> SLQQPEWQSQYAVGLNKLDPHTYVWPYADASEVEKGTFEQSPYYMSLNGQWKFHWVKNPDTRPKDFYKPSYYTGGWADIKVPGNWERQGYGTAIYVNETYEFDDKMFNFKKNPPLVPYKENEVGSYRRTFKVPAGWEGRRVVLCCEGVISFYYVWVNGEFLGYNQGSKTAAEWDITDKLTDGENTIALEVYRWSSGAYLECQDMWRLSGIERDVYLYSTPEQYIADYKVTSLLEKEHYKEGIFELEVAVGGTASGTSSIAYTLKDASDKTVLEGSRKLESHGSGNLIVFDEQRLPDVRRWNAEHPELYTLLLELKDAGGKVTEITGTKVGFRTSEIKNGRFCINGVPVLVKGVNRHEHSQLGRTVSKELMEQDIRLMKQHNINTVRNSHYPAHPYWYQLCDRYGLYVIDEANIESHGMGYGPASLAKDSTWLPAHIDRTRRMYERSKNHPSVVIWSLGNEAGNGINFERTYDWLKSVEKNRPVQYERAEENYNTDIYCRMYRSVDVIRNYVVRKDIYRPFILCEYLHAMGNSCGGMKEYWEVFENEPMAQGGCIWDWVDQSFREVDKDGKWYWTYGGDYGPKDVPSFGNFCCNGLVNAVREPHPHLLEVKKIYQNIKSTLIDKKNLTVRVKNWFDFSDLNEYILHWKVTGDDGTVLAEGNKEVACEPHATVELTLGAVQLPKTIREAYLDLGWTRKKSTPLVDTAWEIAYDQFVLPASGKVWNGKPSEAGKTTFEVDENTGALKSLCLDGEELLASPVTISLFRPATDNDNRDRMGAKLWRKAGLHTLTQKVVSLKESKTSATAQVNILNVTGKKVGDATLEYTLNHNGSLKVQTTFQPDTTWVKSIARLGLTFEMNDTYGNVTYLGRGEHETYIDRNQSGKIGIYTTTPE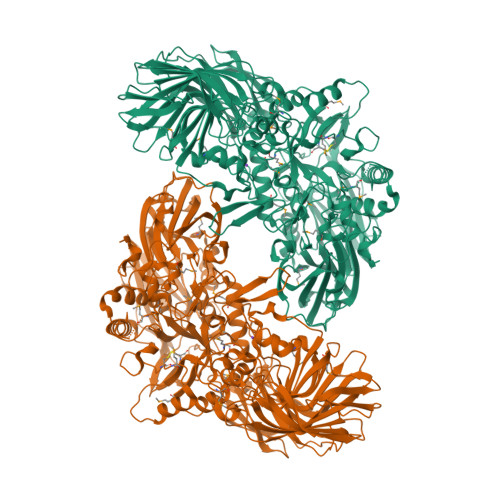KMFHYYVIPQSTGNRTDVRWVKLADDSGKGCWIESDSPFQFSALPFSDLLLEKALHINDLERNGRITVHLDAKQAGVGTATCGPGVLPPYLVPLGKQTFTFTIYPVKEG> MIPINIKDFNYSDPVNNQDIILVKNEKGSFDKGFFVADKILLVPARYGNISTDEGGITSKKEKAHVDKKIYLETDSEKNEYLKNMTTLLKRMNSYSTGNKLLNLIIKGEPIYSKDLQGKFIEQTPSRYLDTNTGKRRVNVMITGPGSNVLTKKCTHNGMGLENDPNGKHSNGTGILSTIEFSPNYLIAYNKCVADPVLTLFHELVHSMHNLYGIAFPDNVKVPYNALKDKNLVSGEEALSEILT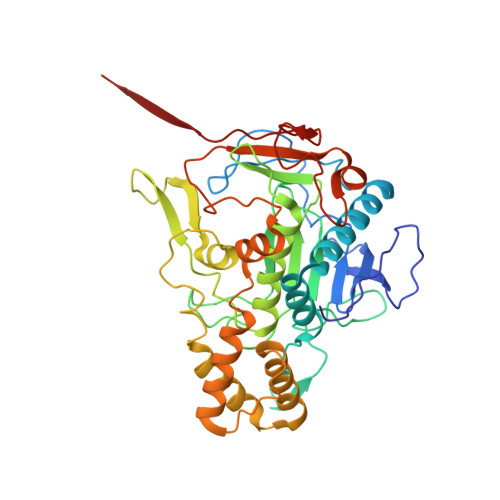FGGKDLTTEHLETLWKKLAETVIIVKDFVKTDTQAKDVFLNNLRFLSKNENIKIDTIEDIVNGTLKIKNNISNLTECEFCKEIGDVRIRTRYAVHSEDVTPVEVVDFKNNYKLNSGFLEGQDISKKYFITNPPKMRRRALRNFKCTIQ>[2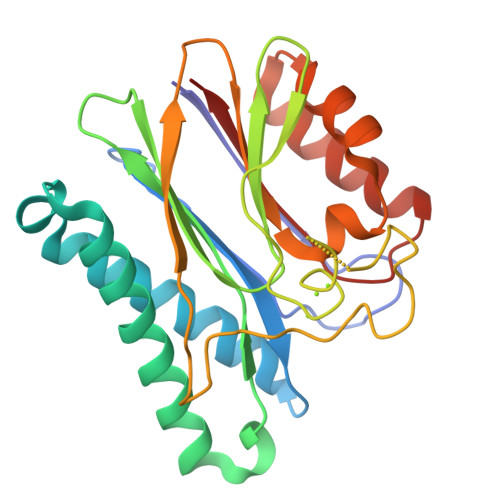x]MDVAGLTDCGLIRKSNQDAFYIDEKHQRFFIVADGMGGHAGGEEASRLAVDHIRQYLETHLEDLQHDPVTLLRQAFLAANHAIVEQQRQNSARADMGTTAVVILLDEKGDRAWCAHVGDSRIYRWRKDQLQQITSDHTWIAQAVQLGSLTIEQARQHPWRHVLSQCLGREDLSQIDIQPIDLEPGDRLLLCSDGLTEELTDDVISIYLSEPNVQKAAAALVDAAKTHGGRDNVTVVVISV> MGFEFTLMVVGESGLGKSTLVNSLFLTDLYPERIIPDAIEKQKQTVKLEASTVEIEERGVKLRLTVVDTPGFGDAIDNSNSFGAILEYIDEQYERFLRDESGLNRRNIVDNRIHCCFYFISPFGHGLKPLDVEFMKKLHSKVNIVPVIAKADCLTKKEILRLKCRIMQEIESHGIKIYPLPDCDSDEDEDYKEQVKQLKEAVPFAVCGANTLLEVKGKKVRGRLYPWGVVEVENPDHCDFIKLRTMLITHMQDLQEVTQEVHYENYRSDRLAKGI;> 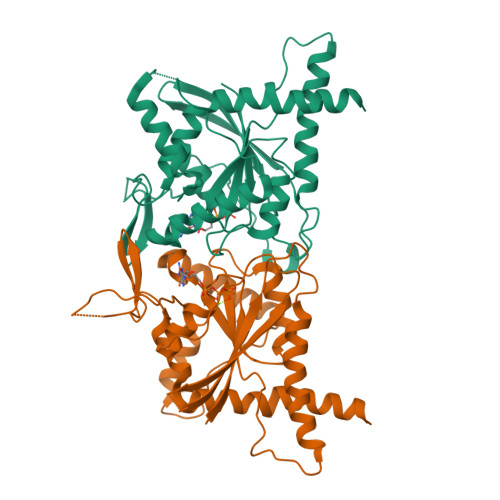MGSSHHHHHHSQDPGFVFNVMCIGETGLGKSTLMDTLFNTSFESTPSPHTLPSVKLKAHTYELQESNVRLKLTICDTVGYGDQINKDDSFKAVVDYIDAQFENYLQEELKIKRSLVTCHDSRIHICLYFICPTGHGLKSLDLVCMKKLDSKVNIIPVIAKADTISKVELQRFKAKIIQELNANGVHIYQFPTDDETVAETNTSMNSHIPFAVVGSTEFIKVGNKLIRARQYPWGTVQVENETHCDFVKLREMLIRTNMEDMREKTHTRHYELYRQKRLEQMG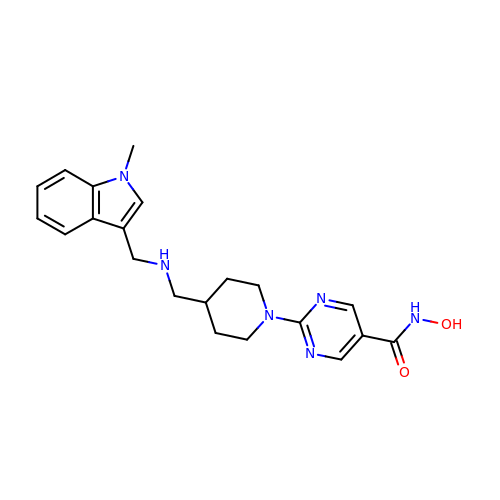2-[4-[[(1-methylindol-3-yl)methylamino]methyl]piperidin-1-yl]-~{N}-oxidanyl-pyrimidine-5-carboxamide | C21 H26 N6 O2 | PAWIYAYFNXQGAP-UHFFFAOYSA-N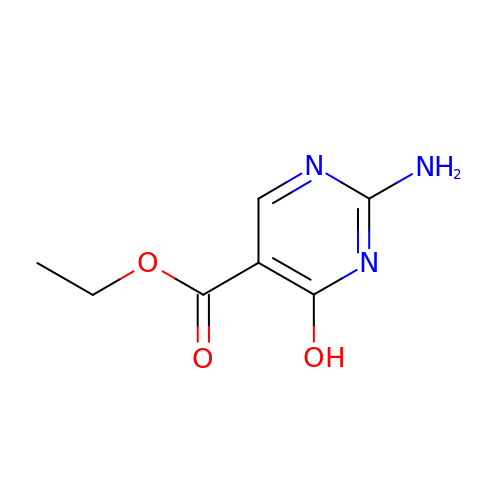2-AMINO-4-HYDROXYPYRIMIDINE-5-CARBOXYLIC ACID ETHYL ESTER | C7 H9 N3 O3 | HRRHGLKNOJHIGY-UHFFFAOYSA-N> MGTIDIITSPTPIHILAFPFPAKGHINPLLHLCNRLASKGFKITLITTVSTLKSVKTSKANGIDIESIPDGIPQEQNHQIITVMEMNMELYFKQFKASAIENTTKLIQKLKTKNPLPKVLIYDSSMPWILEVAHEQGLLGASFFTQPCSVSAIYYHMLQGTIKLPLENSENGMVSLPYLPLLEIKDLPGVQQFEDNSEAVAELLADQFSNIDDVDYVLFNTFDALEIEVVNWMGSKWPILTVGPTAPTSMFFLDKKQKNYEDGRSINYLFETNTEVCMKWLDQREID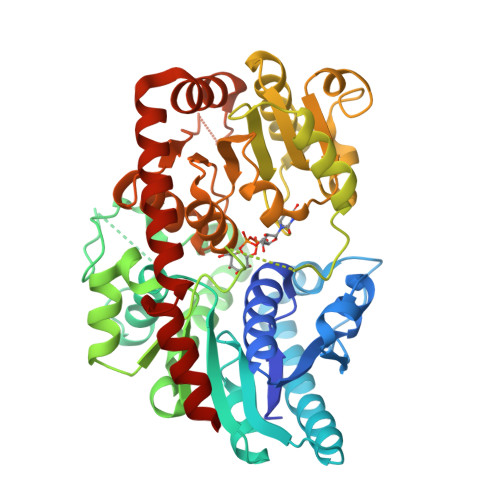TVIYVSFGSLASLTEEQMEQVSQALIRSNCYFLWVVREEEENKLPKDFKETTSKKKGLVINWCPQLDVLAHKSVACFMTHCGWNSTLEALCSGVPMICMPQWADQTTNAKLIEHVWKIGVGVNKSDENGIVKREEIEDCIRQVIESERGKELKRNAIKWKELAKEAVSEGGSSCNNIQEFSSSLLFN> MSKKQPKPVKAEQLKSYYEESRGLERDLIGEFVKSRKTAWRVATASGLFGLLGMVCGIVGFSQPAPAPLVLRVDNATGAVDVVTTLREHESSYGEVVDTYWLNQYV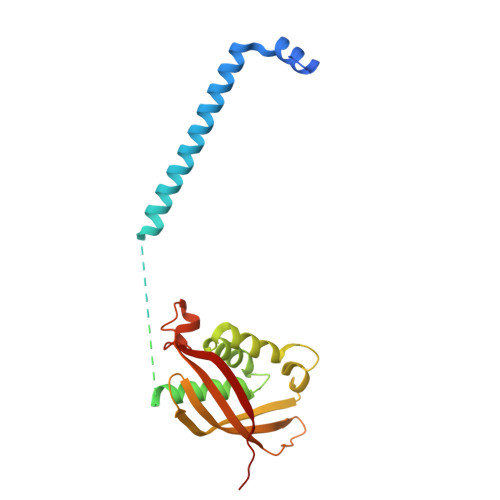LNREAYDYNTIQMNYDTTALLSAPAVQQDYYKLFDGSNARDRVLGNKARITVRVRSIQPNGRGQATVRFTTQQHNSNGTVEAPQHQIATIGYTYIGAPMRSSDRLLNPLGFQVTSYRADPEILNN>[6x]GPHMHKKSFFDKKRSERGSDAGSAGDGASN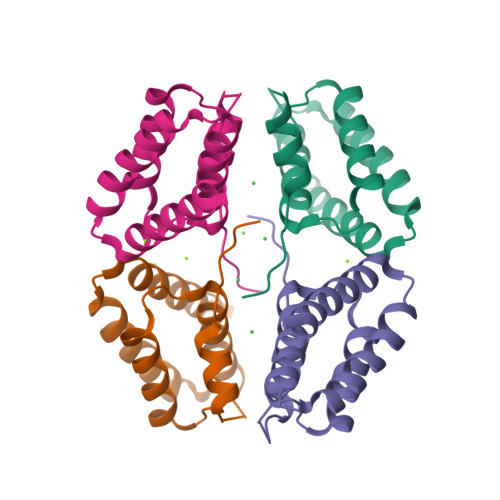LAGAVEFNDVKTLLREWITTISDPMEEDILQVVKYCTDLIEEKDLEKLDLVIKYMKRLMQQSVESVWNMAFDFILDNVQVVLQQ ethyl 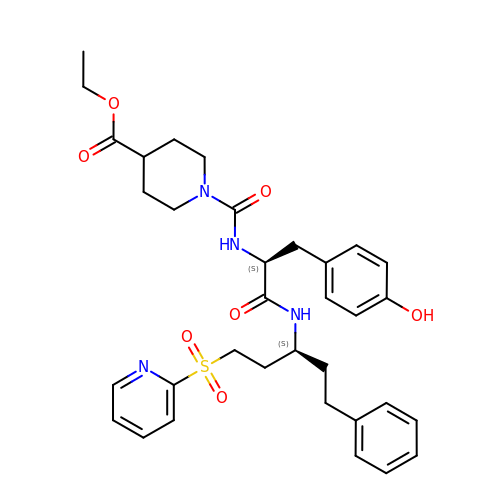1-[[(2~{S})-3-(4-hydroxyphenyl)-1-oxidanylidene-1-[[(3~{S})-1-phenyl-5-pyridin-2-ylsulfonyl-pentan-3-yl]amino]propan-2-yl]carbamoyl]piperidine-4-carboxylate | C34 H42 N4 O7 S | ADLUELBPENMFTG-JDXGNMNLSA-N(3S)-3,7-DIAMINOHEPTANOIC ACID | C7 H16 N2 O2 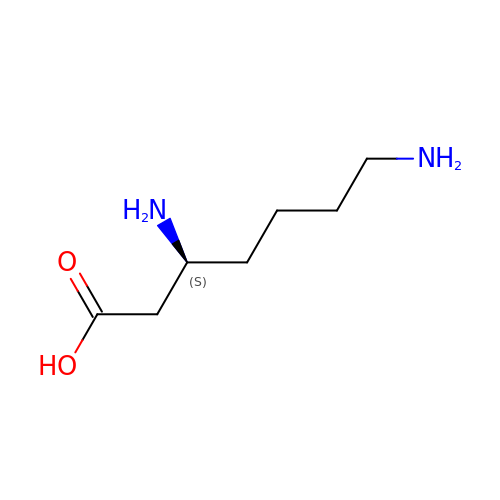| PJDINCOFOROBQW-LURJTMIESA-N Cyanophycin, a nonribosomally synthesized polypeptide consisting of equimolar amounts of aspartate and arginine as the backbone and branched sidechain, respectively, was first identified in cyanobacteria in the form of opaque and light-scattering cytoplasmic granules. The biosynthesis of cyanophycin is achieved by a single enzyme named cyanophycin synthetase (CphA1) that catalyzes peptide elongation coupled with ATP hydrolysis. The discrete active sites of the G and M domains are used for extending the Asp backbone and attaching the Arg sidechain, respectively.

In the cryo-EM map processed with C1 symmetry, all the TeCphA1 protomers in the tetramer bound a cyanophycin primer peptide, (β-Asp-Arg)4, on the surface of Gcore. The cryo-EM map showed a clear density for the C-terminal β-Asp-Arg dipeptide unit (4th unit) and the other Asp backbones with a hook-like shape. Since the Arg sidechains of the 1st and 2nd units were invisible in the cryo-EM map, these models could not be built in the substrate-bound TeCphA1 structure. In the TeCphA1 structure, the C-terminal backbone carboxy group and Arg sidechain of the 4th unit interact with Arg309 (the nearest atomic distance, 2.9 Å) and Glu215, which is derived from another protomer forming the Gcore-Gcore dimer (Glu215’) (2.8 Å), respectively. Since (β-Asp-Arg)4 is well accommodated at the binding site of Gcore, a cyanophycin molecule with at least 3‒4 dipeptides long seems to be suitable as a primer peptide for TeCphA1 activity. In protomers A and B, Mlid and Mcore sandwich ATPγS, and Arg731 and His748 in Mlid interact with the α-phosphate and γ-thiophosphate groups of ATPγS. While ATPγS was visible on all M domains, (β-Asp-Arg)4 was not observed on the M domain of the substrate-bound TeCphA1 structure.

>[4x]MKILKLQTLRGPNYWSIHRHKLVVMRLDLEDLYEKYTSDIPGFYKGLTEVLPSLVEHLCSPGVKGGFLTRVEKGTLIGHVIEHVAIELQELAGMPVGFGRTRETSTTGVFQVVIEYENEQAGRYAARAAVRLCQSIVDTGTYPATELQQDLEDLKELKNQASLGPSTEAIVKEAEARGIPWTQLGARFMIQFGYGVNQKKIQATLSNQTGILGVELACDKEGTKRILKDAGVPVPRGTVARYFDELQDAIEYVGGYPIVIKPLDGNHGRGITIDVKNWQEAEEAYDLARKASKTKTVIVERYYTGKDHRVLVVNGKVVAVAERVPAHVVGNGKSTIAELIEETNRDPQRGDGHDNILTRITVDKSALDILGKQGYSIDSIPLKGKKCFLRATANLSTGGIAVDRTDEIHPENVWLLSRVAKIIGLDIAGIDVVTEDISQPLREVEGVIVEVNAAPGFRMHVAPSRGLARNVAGAVMDMLFPGSKNGRIPILSVTGTNGKTTTTRLLAHIIKQTGKVVGYTTTDGTYIGEYLAETGDNTGPQSAHLILSDPTVEVAVLETARGGILRSGLGFSSCEVGIVLNVTADHLGIGDIDTIEQLAKLKSVVAESVMPKGYAVLNAEDPLVAAMADRVKGQVAYFSMDPNNELLLRHTEAGGLAAIYENGYISILKGDWTLRIEKAVNVPITMAGKAPFMIANALAACLAVFTQGVKIEHIRKGLSTFVASVDQTPGRMNMFNMGSYHALVDYAHNPASYEALGGFVRNWPGKRIGVVGGPGDRRDEDFVSLGELAADIFDEIIIKEDDDTRGRPRGNAAELICQGVKQFLNGIKNSESKATYESILDETAAINTALDRAPIDGLVVILPESVNRAISLIEGRHVIQDIELLQDSQREPKDQEVLKSSILEHHHHHH;>DDDD[4x]>[2x]HHHHHHFNLPPGNYKKPKLLYCSNGGHFLRILPDGTVDGTRDRSDQHIQFQLSAESVGEVYIKSTETGQYLAMDTDGLLYGSQTPNEETLFLERLEENHYN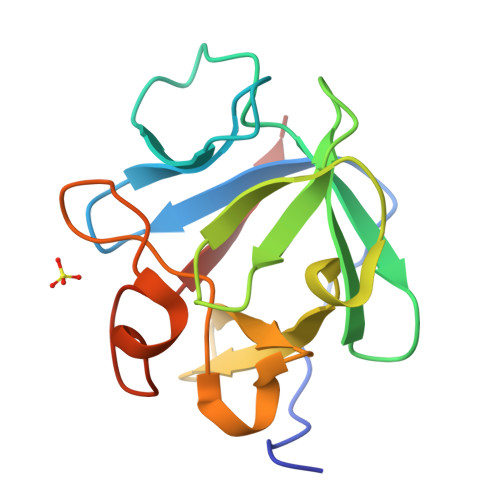TYISKKHAEKNWFVGLKKNGSVKRGPRTHYGQKAILWLPLPVSSD>KPQVTILATGGTIAGSGESSVKSSYSAGAVTVDKLLAAVPAINDLATIKGEQISSIGSQEMTGKVWLKLAKRVNELLAQKETEAVIITHGTDTMEETAFFLNLTVKSQKPVVLVGAMRPGSSMSADGPMNLYNAVNVAINKASTNKGVVIVMNDEIHAAREATKLNTTAVNAFASPNTGKIGTVYYGKVEYFTQSVRPHTLASEFDISKIEELPRVDILYAHPDDTDVLVNAALQAGAKGIIHAGMGNGNPFPLTQNALEKAAKSGVVVARSSRVGSGSTTQEAEVDDKKLGFVATESLNP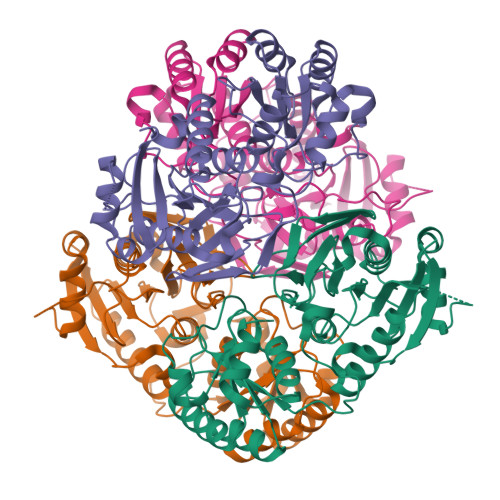QKARVLLMLALTKTSDREAIQKIFSTY[4x]>HHAIGYVWNTLYGWVDTGTGSLAAANLTARMQPISHHLAHPDTKRRFHELVCASGQIEHLTPIAAVAATDADILRAHSAAHLENMKRVSNLPTGGDTGDGITMMGNGGLEIARLSAGGAVELTRRVATGELSAGYALVNPPGHHAPHNAAMGFCIFNNTSVAAGYARAVLGMERVAILDWDVHHGNGTQDIWWNDPSVLTISLHQHLCFPPDSGYSTERGAGNGHGYNINVPLPPGSGNAAYLHAMDQVVLPALRAYRPQLIIVGSGFDASMLDPLARMMVTADGFRQMARRTIDCAADICDGRIVFVQEGGYSPHYLPFCGLAVIEELTGVRSLPDPYHE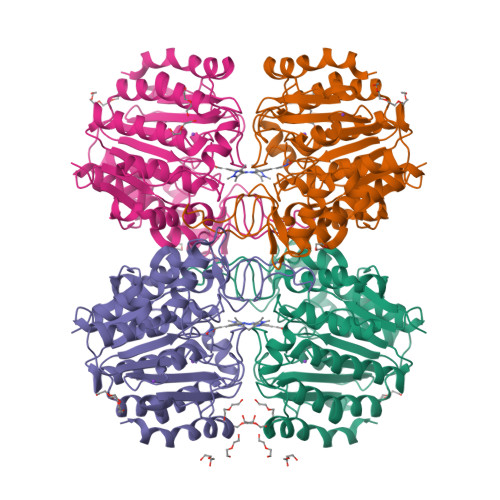FLAGMGGNTLLDAERAAIEEIVPLLADIR[2x]> HGSPVDICTAKPRDIPMNPMCIYRSPEKKATEDEGSEQKIPEATNRRVWELSKANSRFATTFYQHLADSKNDNDNIFLSPLSISTAFAMTKLGACNDTLQQLMEVFKFDTISEKTSDQIHFFFAKLNCRLYRKAAKSSKLVSANRLFGDKSLTFNETYQDISELVYGAKLQPLDFKENAEQSRAAINKWVSNKTEGRITDVIPSEAINELTVLVLVNTIYFKGLWKSKFSPENTRKELFYKADGESCSASMMYQEGKFRYRRVAEGTQVLELPFKGDDITMVLILPKPEKSLAKVEKELTPEVLQEWLDELEEMMLVVHMPRFRIEDGFSLKEQLQDMGLVDLFSPEKSKLPGIVAEGRDDLYVSDAFHKAFLEVNEEGAEAAASTAVVIAGRSLNPNRVTFKANRPFLVFIREVPLNTIIFMGRVANPCVK;> HGSPVDICTAKPRDIPMNPMCIYRSPEKKATEDEGSEQKIPEATNRRVWELSKANSRFATTFYQHLADSKNDNDNIFLSPLSISTAFAMTKLGACNDTLQQLMEVFKFDTISEKTSDQIHFFFAKLNCRLYRKANKSSKLVSANRLFGDKSLTFNETYQDISELVYGAKLQPLDFKENAEQSRAAINKWVSNKTEGRITDVIPSEAINELT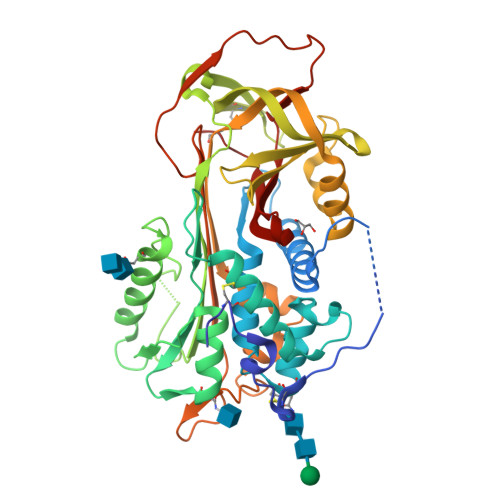VLVLVNTIYFKGLWKSKFSPENTRKELFYKADGESCSASMMYQEGKFRYRRVAEGTQVLELPFKGDDITMVLILPKPEKSLAKVEKELTPEVLQEWLDELEEMMLVVHMPRFRIEDGFSLKEQLQDMGLVDLFSPEKSKLPGIVAEGRDDLYVSDAFHKAFLEVNEEGSEAAASTAVVIAGRSLNPNRVTFKANRPFLVFIREVPLNTIIFMGRVANPCVK> MNIFRLTGDLSHLAAIIILLLKIWKSRSCAGISGKSQLLFALVFTTRYLDLFTSFISLYNTSMKLIYIACSYATVYLIYMKFKATYDGNHDTFRVEFLIVPVGGLSFLVNHDFSPLEILWTFSIYLESVAILPQLFMISKTGEAETITTHYLFFLGLYRALYLVNWIWRYYFEGFFDLIAVVAGVVQTVLYCDFFYLYVTKV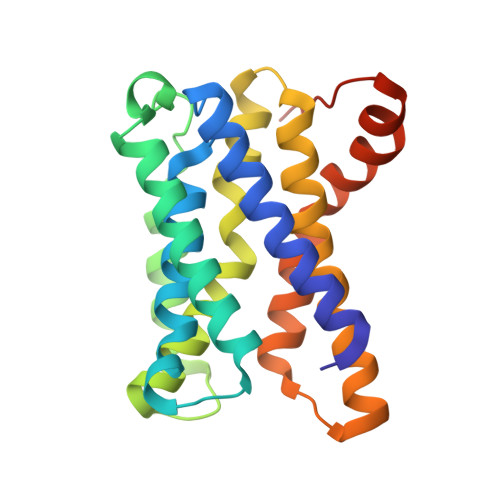LKGKKLSLPAGENLYFQ>MTIKTFLPKKIRGIALLTVSVLSVVMIPVAQSQLVFRNTVTGDVLDLSFGKKGEKTEAVEHFLNTGENLYNTDD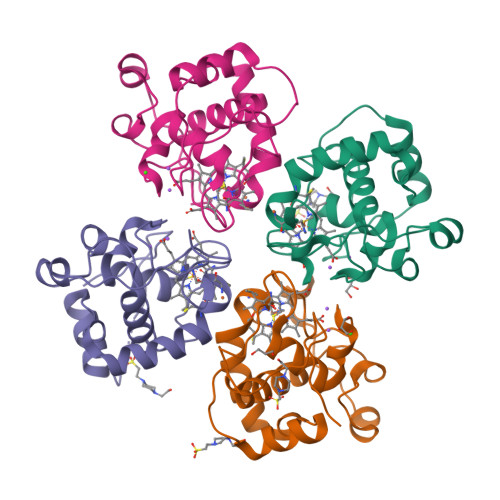EAIKAGESLFMTACSGCHGHHAEGKLGPALGDDYYTYPKNANDKGLFETIYGGARSMMGPQYNNLTKDEILHIMAWVRSVYWGSADKADWLTEEQKANFKPAEVPEDFKEAMDNFNKTHH[4x]Bacterial hybrid malic enzymes (MaeB grouping, multidomain) catalyse the transformation of malate to pyruvate, and are a major contributor to cellular reducing power and carbon flux. Distinct from other malic enzyme subtypes, the hybrid enzymes are regulated by acetyl-CoA, a molecular indicator of the metabolic state of the cell. The larger ME isoforms (hybrid enzymes) are predicted to be a fusion of two unrelated enzymes; a catalytic N-terminal ME subunit and a C-terminal phosphotransacetylase (PTA) domain. The PTA domain is homologous to PTA enzymes (that interconvert acetyl-CoA and phosphate to CoA and acetyl phosphate), yet they appear to lack critical catalytic residues and thus acts as a sensor instead.

We used our Br−/urea protocol to successfully obtain a full-length apoprotein, MaeBapo, from which we were able to determine a crystal structure at 3.70 Å resolution. Despite the limited resolution of this dataset, the electron density is readily interpretable, with good refinement statistics. The structure was not solvable using the MaeBbound full-length model, necessitating the use of isolated MaeBME and MaeBPTA search models, which results from large conformational differences between MaeBbound and MaeBapo. MaeBapo preserves the hexameric D3 symmetry of MaeBbound, but completely changes the placement of the ME dimer. Loss of acetyl-CoA causes a dramatic change to the ME:PTA domain relationship, mediated via a remodelling of the L1:L2 helix interaction. In MaeBapo, L1 sits directly under L2 (helices in the same plane), replacing interactions made by the hook region in MaeBbound (helices ~120° apart). Thus, the MaeBapo structure reveals a requirement for L1:L2 complementarity, with hydrophobic contacts at the interhelical turn (A434:V441) and polar contacts along the helical faces (R444 and N448 to D426/E430/E433). Dyndom analysis reveals that the apo to bound transition is represented by a 69° relative rotation of the ME dimer, with a 3.4 Å translation that pulls the ME dimer away from the PTA regulatory hub. Resulting from this large-scale rotation, the ME hook subdomain is freed from the clash with L2 observed in MaeBbound, and is now located under PTA d1 where it is able to adopt a helical conformation identical to that determined for the isolated ME domain structure. The net effect of this rotation is to “pull” the ME dimer into alignment with the PTA dimer, resulting in a thinner/streamlined hexamer, 74 Å wide versus 90 for the bound state.

>[3x]MGSSHHHHHHSMDNKTETKIEPKTGTTNFDQEALLYHQQGKPGKIEVISSKPCATEKDLSLAYSPGVAAPCKAIAKDPAKVYDYTAKGNLVAVISNGTAVLGLGNIGPAAGKPVMEGKGILFKQFAGIDVFDIEVAATDVDVFCNAVRVLEPTFGGINLEDIKAPECFEIEERLKKEMNIPVFHDDQHGTAIVSGAALLNACSITNRKMETVRIVVNGAGASANSCAKIFIALGARRENIIMCDSQGVIYKGRTAGMNKYKEYFASETEARTLTEALRGADVFVGLSVAGALTPEMLKDMAKDPIIFAMANPEPEITPDKARAARPDAIIATGRSDYPNQVNNVLGFPSIFRGALDTRSTQINEEMKLAAVHALAKLAREDVPDKVSATYGGKSFKFGRDYLIPKPFDTRVLLWVAPEVAKAAMKSGVATRAIEDWDQYRESLEALQGPSKVFIRSAINRVHQNSAANGGELPRIVFPEGTSTKVLKALATLVEEKICQPILLGYPERVKEKIKALDIPLLNDVSIVHPSSHPKYFSFVEKLYSLRQRKGINLGEAERLMADPNYFAAMMVNQGEADGMVSGSSINYADAVRPILQTIGVYKEGIPAGLNFVLLEDKFLVLADTTVNLNPTAEQCAQIALQAAKIVEYFGIEPRVAMLSYSNFSGAEGTPRKMKKAAEIARSLRPDLMIEGDMQADTAVNPEIMERLFPFSGLKGGANVLVFPNLESSNIAYKLIQQIGKAEVIGPFLTGVRRSANVLQRTTTVDGIVNSVVFTALEAQYIKEVLKSRGKK> MAHHHHHHMNPHPVEPRDQIAELLVESPLFSFNCAHFIAFKGFRATLHGHNYNVSLRLRGNIQGDGYVIDFSILKEKVRKVCKQLDHHFILPMYSDVLNIQEVNDNFKITCEDNSEYS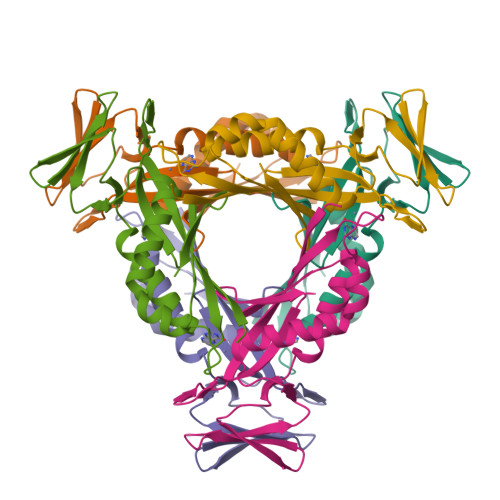FPKRDCVQIPIKHSSTEEIGLYILNQLIEEIDLPFLKTRSVNYMEVTVSESPSQKATVHRNI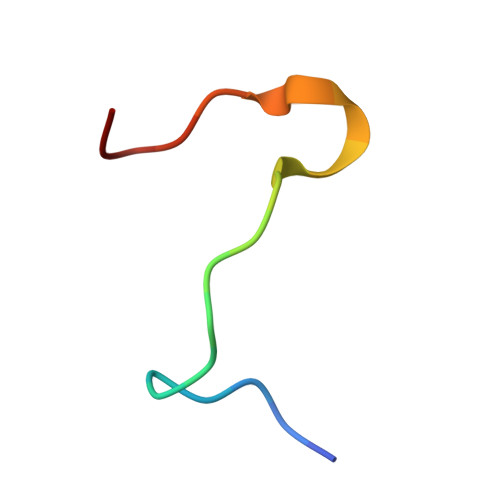> RHVSSSDRVGKPYRGVKPVFS> MASNAARVVATAKDFDKVGLGIIGYYLQLYAVELILSEEDRSQEMTALATELLDTIEAFKKEIGGESEAEDSDKSLHVMNTLIHDQEKAKIYMLNFTMSLYNEKLKQLKDGPWDVMLKRSLWCCIDLFSCILHLWKENI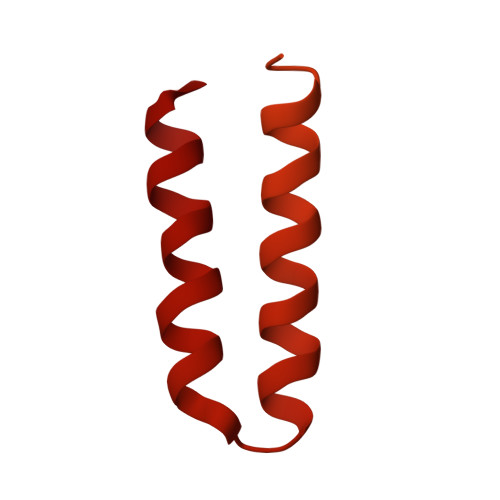SETSTNSLQKRIKYCKIYLSKLAKGEIGSSDEKTLDYADFADDSEEIKDEDVDHQTSDLENNNNDKVEGLAPKDQTTSYEPVDEVPEFIDDADSVNEEEQTVDKNEDAITKDEQQVVKKEVDLTRPSAPSEPAAAEHKSYTKDELTKIMDRASKIEQIQKLAKYAISALNYEDLPTAKDELTKALDLLNSI>[4x]MARIPYKVAVIGTGRVGATFAYTMAVVPGIARMTLVDVVPGLAKGVMEDIKHAAAVFRRSITVEAFEDVSKVENADAIVITAGKPRKADMSRRDLANVNAQIIRDIGDKLRDRNPGALYVVVTNPVDVMTMVLDDVIGSKGTVIGTGTSLDTFRFRAAVSELLNVPIVAVDGYVVGEHGEEAFVAWSTVTIKGIHIDQYIKERNINISREQIEKYVKDVAASIIASQGATIWGPAAT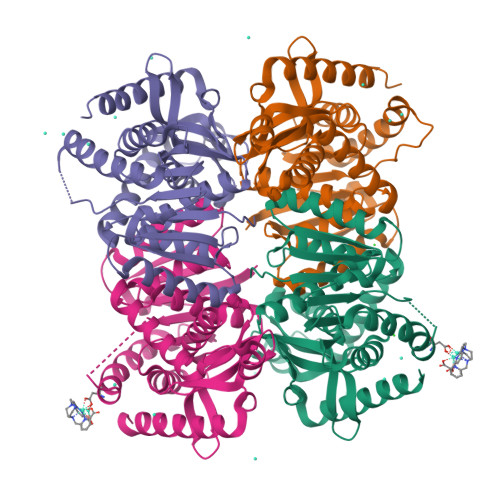FQEIVVSHLANESKIIPISLPQNIEGVGRVAVSVPTIISGRLKPLVQLLNEEEQERLKRAAKAIRNVYESILT> PPGTPSRHEKSLGLLTTKFVSLLQEAKDGVLDLKLAADTLAVRQKRRIYDITNVLEGIGLIEKKSKNSIQWKGVGP;> RSKKGDKNGKGLRHFSMKVCE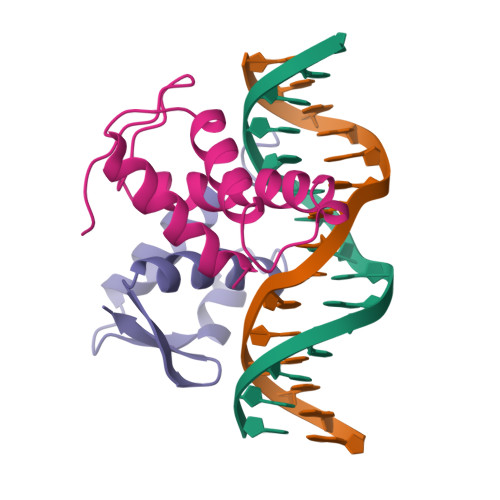KVQRKGTTSYNEVADELVSEFTNSNNHLAADSAYDQKNIRRRVYDALNVLMAMNIISKEKKEIKWIGLPTNSAQ>MALLTPIPSPMVNLTQVIDPTEQLAYFPKITFERLKNYDTSSNYAKGKLTRNYMILLPWQHVNRYNFVFSSTGCKVSLKTCIGKLMKDLNPKVLYFIGEGAGNWMARTACEYPDIKFVYRSLKDDLDHHYPLEYQRVIGELSRIIDSGEGLSMETTDATQKTHWDLIHRVSKDALLITLCDAEFKDRDDFFKMVILWRKHVLSCRICTTYGTDLYLFAKYHAKDCNVKLPFFVRSVATFIMQGSKLSGSECYILLTLGHHNNLPCHGEIQNSKMKIAVCNDFYAAKKLDNKSIEANCKSLLSGLRIPINKKELNRQRRLLTLQSNHSSVATVGGSKVIESKWLTNKANTIIDWLEHILNSPKGELNYDFFEALENTYPNMIKLIDNLGNAEIKKLIKVTGYMLVSKKSGHHHHHH[2x]

The Mononegavirales order groups five families of monopartite, negative-strand RNA viruses many of which are highly pathogenic and/or contagious; the Filoviridae (of which Ebola virus is a representative), the Bornaviridae (Borna disease virus), the Nyamiviridae (midway virus), the Rhabdoviridae (rabies, vesicular stomatitis virus (VSV)) and the Paramyxoviridae (measles virus, human metapneumovirus (hMPV)). These viruses encode a large RNA polymerase (L) (usually >2,000 amino acids) that is crucial to viral replication. As a part of this study, we expressed CR-VI+, a 406-residue fragment comprising CR-VI and the adjoining ‘+ domain’, the variable region carrying the K-K-G-motif, investigated its MTase activity and solved its crystal structure. Besides sequentially methylating the 2′O and N7 atoms of small capped RNAs, CR-VI+ also 2′O methylates uncapped substrates and displays nucleotide triphosphatase (NTPase) activity. Both the CR-VI domain, which assumes a fairly standard MTase fold, and the K-K-G motif of the (mainly helical) +domain are required for the MTase reactions.

Most notably, hMPV and flaviviruses share an unusually long (∼10 residues), flexible β2λ (that is, the loop immediately following the β2-strand), which forms the SAM-binding pocket (SAMP) along with loops β1λ and β4λ, shielding it from the solvent. In CR-VI+, β2λ similarly assumes alternate conformations. Loops β1λ and β4λ also show a degree of flexibility. β1λ residue E1697, conserved in paramyxo- and filoviruses, forms a hydrogen bond with the NH2 group of SAM and is essential for both MTase activities. However, in the absence of SAM, its side chain either moves into the sub-pocket that normally accommodates the NH2 group, or, more markedly, turns towards the solvent in the direction of β2λ, which in this case assumes the ‘open’ position. β4λ forms a side wall of SAMP, and together with αD and β5 also defines a deep, hydrophobic cavity not present in other MTases, termed NSP (or nucleoside-binding pocket).> MKKAVINGEQIRSISDLHQTLKKELALPEYYGENLDALWDC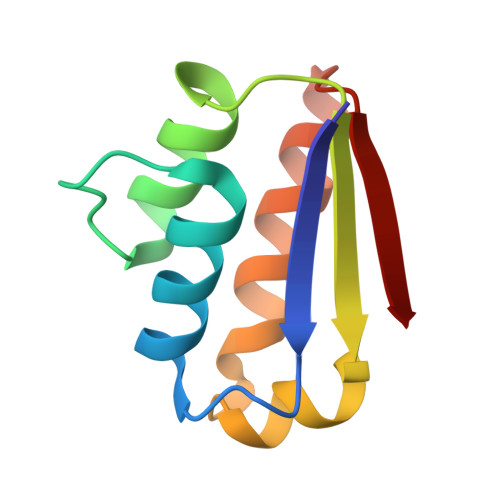LTGWVEYPLVLEWRQFEQSKQLTENGAESVLQVFREAKAEGCDITIILS>[4x]AMGSRLYDRRSIFDAVAQSNCQELESLLPFLQRSKKRLTDSEFKDPETGKTCLLKAMLNLHNGQNDTIALLLDVARKTDSLKQFVNASYTDSYY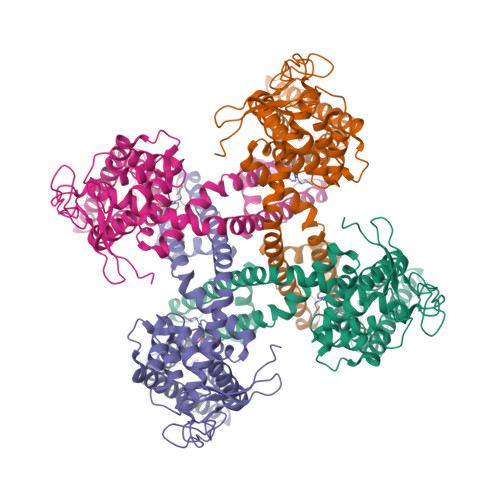KGQTALHIAIERRNMTLVTLLVENGADVQAAANGDFFKKTKGRPGFYFGELPLSLAACTNQLAIVKFLLQNSWQPADISARDSVGNTVLHALVEVADNTVDNTKFVTSMYNEILILGAKLHPTLKLEEITNRKGLTPLALAASSGKIGVLAYILQREIHEPECRHLSRKFTEWAYGPVHSSLYDLSCIDTCEKNSVLEVIAYSSSETPNRHDMLLVEPLNRLLQDKWDRFVKRIFYFNFFVYCLYMIIFTAAAYYRPVEGLPPYKLKNTVGDYFRVTGEILSVSGGVYFFFRGIQYFLQRRPSLKSLFVDSYSEILFFVQSLFMLVSVVLYFSQRKEYVASMVFSLAMGWTNMLYYTRGFQQMGIYAVMIEKMILRDLCRFMFVYLVFLFGFSTAVVTLIEDGKYNSLYSTCLELFKFTIGMGDLEFTENYDFKAVFIILLLAYVILTYILLLNMLIALMGETVNKIAQESKNIWKLQRAITILDTEKSFLKCMRKAFRSGKLLQVGFTPDGKDDYRWCFRVDEVNWTTWNTNVGIINEDPG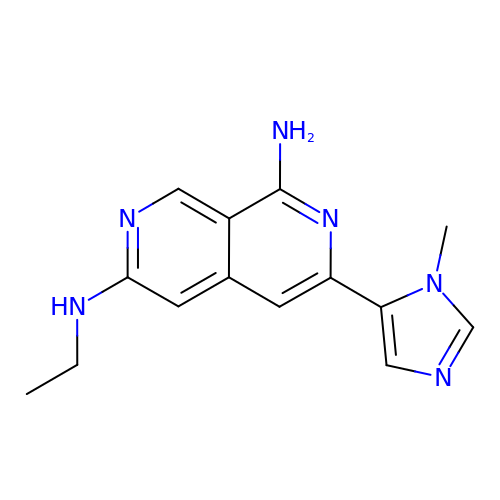(3M)-N~6~-ethyl-3-(1-methyl-1H-imidazol-5-yl)-2,7-naphthyridine-1,6-diamine | C14 H16 N6 | ZZRQLAUQECWGOR-UHFFFAOYSA-N>[2x]GMSISSKAKEILTQFTREVWSEGNIE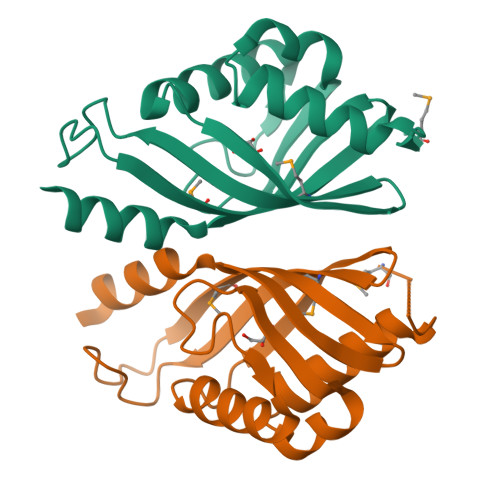ASDKYIAPKYTVLHDPGDPWEGRELDVAGYKERVKTLRAAFPDQCFDIQGLFADGDAVVMTWLWTATHKEDIPGFPSTGKQIKMSGATVYYFDGNRLTGHWQITDRLGVYQQLRQAAAGA>[4x]GPGSGTMLPVFCVVEHYENAIEYDCKEEHAEFVLVRKDMLFN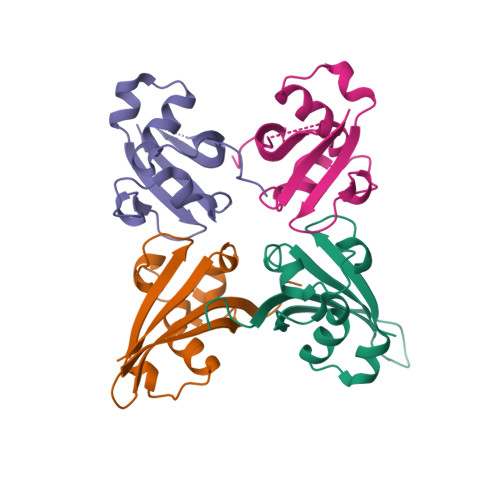QLIEMALLSLGYSHSSAAQAKGLIQVGKWNPVPLSYVTDAPDATVADMLQDVYHVVTLKIQLH> MA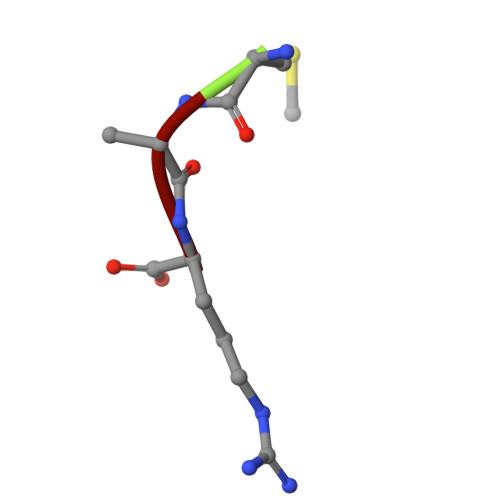R> VKVQPNDYVFRDLANHNQIFVKDKDPKVYNNPYYIDQVQLKDAQQTDLTSIQASFTTLDGVDKTEILKELKVTDKNQNAIQISDITLDTSKSLLIIKGDFNPKQGHFNISYNGNNVTTRQSWEFKDQLYAYSGNLGAVLNQDGSKVEASLWSPSADSVTMIIYDKDNQNRVVATTPLVKNNKGVWQTILDTKLGIKNYTGYYYLYEIKRGKDKVKILDPYAKSLAEWDSNTVNDDIKTAKAAFVNPSQLGPQNLSFAKIANFKGRQDAVIYEAHVRDFTSDQSLDGKLKNQLGTFAAFSEKLDYLQKLGVTHIQLLPVLSYFYVNEMDKSRSTAYTSSDNNYNWGYDPQSYFALSGMYSEKPKDPSARIAELKQLIHDIHKRGMGVILDVVYNHTAKTYLFEDIEPNYYHFMNEDGSPRESFGGGRLGTTHAMSRRVLVDSIKYLTSEFKVDGFRFDMMGDHDAAAIELAYKEAKAINPNMIMIGEGWRTFQGDQGKPVKPADQDWMKSTDTVGVFSDDIRNSLKSGFPNEGTPAFITGGPQSLQGIFKNIKAQPGNFEADSPGDVVQYIAAHDNLTLHDVIAKSINKDPKVAEEDIHRRLRLGNVMILTSQGTAFIHSGQEYGRTKRLLNPDYMTKVSDDKLPNKATLIEAVKEYPYFIHDSYDSSDAINHFDWAAATDNNKHPISTKTQAYTAGLITLRRSTDAFRKLSKAEIDREVSLITEVGQGDIKEKDLVIAYQTIDSKGDIYAVFVNADSKARNVLLGEKYKHLLKGQVIVDADQAGIKPISTPRGVHFEKDSLLIDPLTAIVIKVGKVAPSPKEELQADYPKTQSFKGSKTVEKVNRIANKTSITPVVSNKTDSYLTNEANL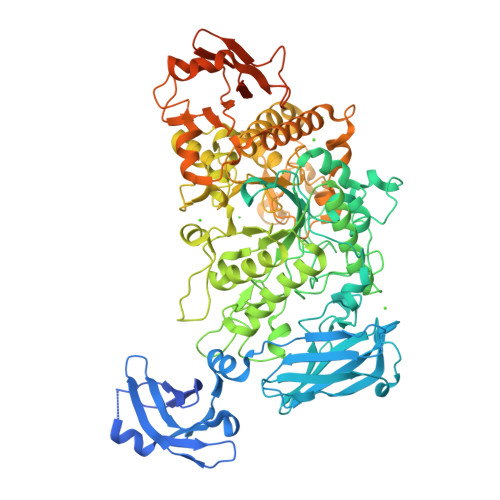EHHHHHH>GGSLNATFYAGTCPNASAMVRTIVQQAFQSDSRIGASLIRLHFHDCFVLGCDASILLDNSGSII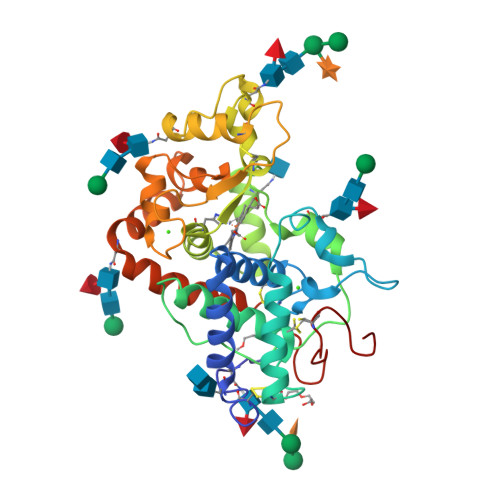SEKNAGPNANSARGFNVVDNIKTALENACPGVVSCTDVLALASQASVSLSGGPSWTVDLGRRDTLTANQAGANSSIPSPTQGLSNITSKFSAVGLNTNDLVALSGAHTFGRATCGVFSNRLFNFSGKGNPDPTLNTTLLSTLQELCPQKGRGSGSTNLDLSTPDAFDNNYFTNLQSNNGLLQSDQELFSTTGSATIAIVTSFASNQTLFFQAFAQSMINMGNISPLTGSSGEIRLDCKKTNGSG[2x]>[2x]SNAMTREATIRQILVITDGCSNIGPDPVEAARRAHRHGIVVNVIGIVGRGDAGEQGYQEAHSIADAGGGMCRIVQPADISATAQMMTHQTMQMTLQQVVNQELLAVMGKSTE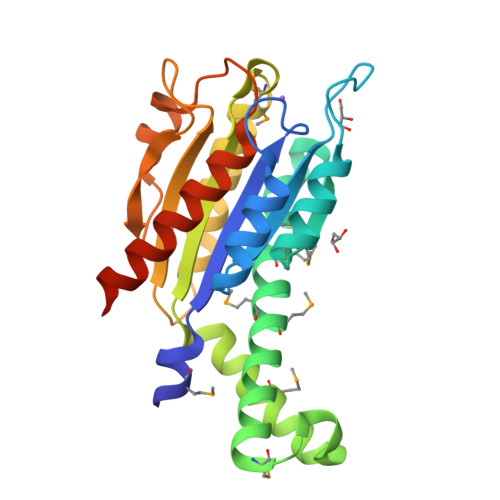DLPPADRARVMQVVEKLEDEVALHLVVCLDTSASMRDKIPTVREAVRDLALSLKVRSGPLAVSVIAFPGKGEEATRLVQPFSSEVNVAALEAELVARGGTPTGPAIDHAADLLLSHARNVDEDAPRREFG>[2x]MSQRITIDPVTRIEGHLRIDCEIENGVVSKAWASGTMWRGMEEIVKNRDPRDAWMIVQRICGVCTTTHAISSVRAAESALNIDVPVNAQYIRNIILAAHTTHDHIVHFYQLSALDWVDITSALKADPAKASAMLNGVSTWHLNSAEEFTKVQNKIKDLVASGQLGIFANGCWGHPAMQLPPEVNLIAVAHYLQALECQRDANRVVALLGGKTPHIQ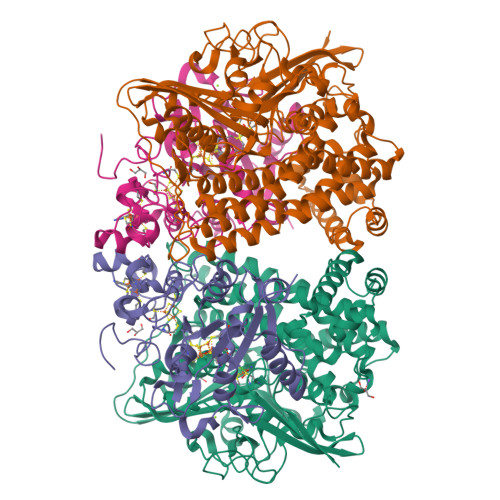NLAVGGVANPINLDGLGVLNLERLMYIKSFIDKLSDFVEQVYKVDTAVIAAFYPEWLERGQGAVNYLSAPEFPTDGKNGSFLFPGGYITDADLSTYRPITSHSDEYLIKGIQESAKHAWYKDEAPQAPWEGTTVPDYTGWSDDGKYSWVKAPTFYGKTVEVGPLANMLCKLAAKRESTHAKLNEIVAIYTKLTGKTIEVAQLHSTLGRIIGRTVHCCELQNVLQDQYNALIVNIGKGDHTTFVKPDIPATGEFKGVGFLEAPRGMLSHWMVIKDGIISNYQAVVPSTWNSGPRNFNDEVGPYERSLVGTPIADPNKPLEVVRTIHSFDPCMSCAVH;>EMAESVSRPQRPPVIWIGAQECTGCTESLLRATHPTVENLVLETISLEYHEVLSAAFGHQVEENKHNALEKYKGQYVLVVDGSIPLKDNGIYCMVAGEPIVDHIRRAAEGAAAIIAIGSCAAWGGVAAAGVNPTGAVGLQEVLPGKTIINIPGCPPNPHNFLATVAHIITYGKPPKLDAKNRPTFAYGRLIHEHCERRPHFDAGRFAKEFGDEGHREGWCLYHLGCKGPETYGNCSTLQFCDVGGVWPVAIGHPCYGCNEEGIGFHKGIHQLAHVENQTPRSEKPDVNIKEGGNISAGAVGLLGGVVGLVAGVSVMAVRELGRQQKKDNADSRGE[2x]> MSALCDPPGAPGPPGPAPATHGPAPLSAQELSQEIKAFLTGVDPILGHQL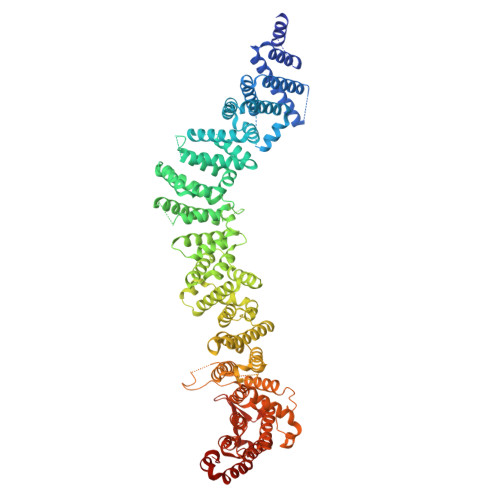SAREHARCGLLLLRSLPPARAAVLDHLRGVFDESVRAHLAALDETPVAGPPHLRPPPPSHVPAGGPGLEDVVQEVQQVLSEFIRANPKAWAPVISAWSIDLMGQLSSTYSGQHQRVPHATGALNELLQLWMGCRATRTLMDIYVQCLSALIGSCPDACVDALLDTSVQHSPHFDWVVAHIGSSFPGTIISRVLSCGLKDFCVHGGAGGGAGSSGGSSSQTPSTDPFPGSPAIPAEKRVPKIASVVGILGHLASRHGDSIRRELLRMFHDSLAGGSGGRSGDPSLQATVPFLLQLAVMSPALLGTVSGELVDCLKPPAVLSQLQQHLQGFPREELDNMLNLAVHLVSQASGAGAYRLLQFLVDTAMPASVITTQGLAVPDTVREACDRLIQLLLLHLQKLVHHRGGSPGEGVLGPPPPPRLVPFLDALKNHVGELCGETLRLERKRFLWQHQLLGLLSVYTRPSCGPEALGHLLSRARSPEELSLATQLYAGLVVSLSGLLPLAFRSCLARVHAGTLQPPFTARFLRNLALLVGWEQQGGEGPAALGAHFGESASAHLSDLAPLLLHPEEEVAEAAASLLAICPFPSEALSPSQLLGLVRAGVHRFFASLRLHGPPGVASACQLLTRLSQTSPAGLKAVLQLLVEGALHRGNTELFGGQVDGDNETLSVVSASLASASLLDTNRRHTAAVPGPGGIWSVFHAGVIGRGLKPPKFVQSRNQQEVIYNTQSLLSLLVHCCSAPGGTECGECWGAPILSPEAAKAVAVTLVESVCPDAAGAELAWPPEEHARATVERDLRIGRRFREQPLLFELLKLVAAAPPALCYCSVLLRGLLAALLGHWEASRHPDTTHSPWHLEASCTLVAVMAEGSLLPPALGNMHEVFSQLAPFEVRLLLLSVWGFLREHGPLPQKFIFQSERGRFIRDFSREGGGEGGPHLAVLHSVLHRNIDRLGLFSGRFQAPSPSTLLRQGT>[2x]GSCPSQCSCSGTDVNCDGARFASVPAAIPI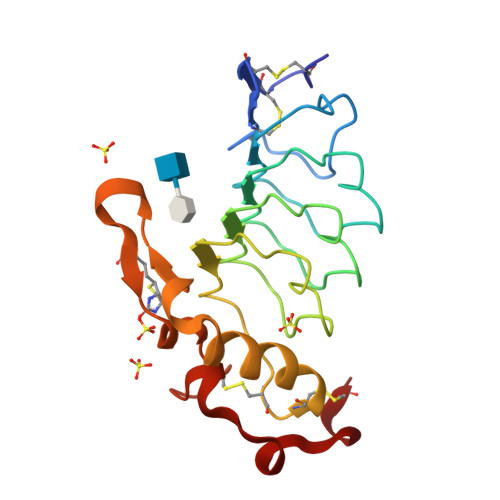TTQRLWLSNNQLTKLDPGVFDSLTQLTTLYLSNNQLTALPAGVFDKLTQLKELGLDQNQLKSIPDGAFARLPSLTHVWLHTNPWDCQCTDILYLSGWVAQHSSIVGEGWLRSWTVNPDNAKCSGTNTPVRAVTEASTSPSKCP> GRGGSSTDQPVANPYNTKEISLAAGLVQQTYCDSTENGLKIGDSELLYTMGEGYARQRVNIYHSPSLGIAVAIEGTNLFSLNSDLHDAKFWQEDPNERYIQYYPKGTKLMHGFQQAYNDLMDDIFTAVKKYKKEKNEKRVTVIGHSLGAAMGLLCAMDIELRMDGGL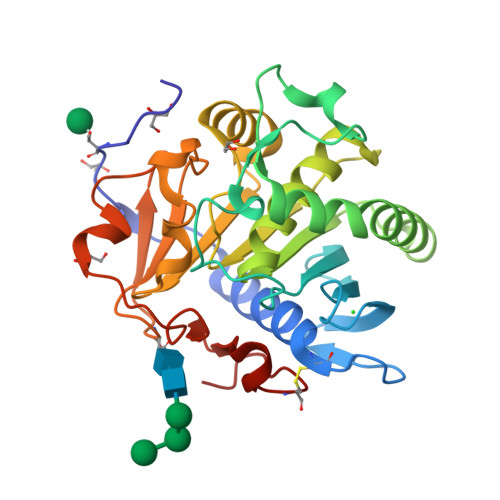YKTYLFGLPRLGNPTFASFVDQKIGDKFHSIINGRDWVPTVPPRALGYQHPSDYVWIYPGNSTSAKLYPGQENVHGILTVAREFNFDDHQGIYFHTQIGAVMGECPAQVGAH> GSSEAKAPTALERVQKEGVLRVITRNSPATYFQD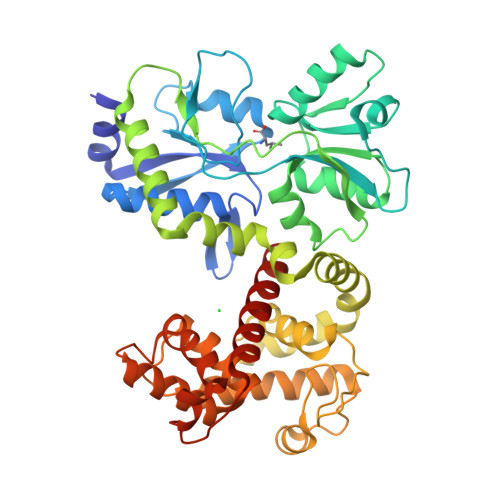RNGETGFEYELAKRFAERLGVELKIETADNLDDLYAQLSREGGPALAAAGLTPGAAADASVRYSHTYLDVTPQIIYRNGQQRPTRPEDLVGKRIMVLKGSSHAEQLAELKKQYPELKYEESDAVEVVDLLRMVDVGDIDLTLVDSNELAMNQVYFPNVRVAFDFGEARGLAWALPGGDDDSLMNEVNAFLDQAKKEGLLQRLKDRYYGHVDVLGYVGAYTFAQHLQQRLPRYESHFKQSGKQLDTDWRLLAAIGYQESLWQPGATSKTGVRGLMMLTNRTAQAMGVSNRLDPKQSIQGGSKYFVQIRSELPESIKEPDRSWFALAAYNIGGAHLEDARKMAEKEGLNPNKWLDVKKMLPRLAQKQWYAKTRYGYARGGETVHFVQNVRRYYDILTWVTQPQ>STGEEVVIAGMSGKLPESENLQEFWDNLIGGVDMVTDDDRRWKAGLYGLPRRSGKLKDLSRFDASFFGVHPKQAHTMDPQLRLLLEVTYEAIVDGGINPDSLRGTHTGVWVGVSGSETSEALSRDPETLVGYSMVGCQRAMMANRLSFFFDFRGPSIALDTACSSSLMALQNAYQAIHSGQCPAAIVGGINVLLKPNTSVQFLRLGMLSPEGTCKAFDTAGNGYCRSEGVVAVLLTKKSLARRVYATILNAGTNTDGFKEQGVTFPSGDIQEQLIRSLYQSAGVAPESFEYIEAHGTGTKVGDPQELNGITRALCATRQEPLLIGSTKSNMGHPEPASGLAALAKVLLSLEHGLWAPNLHFHSPNPEIPALLDGRLQVVDQPLPVRGGNVGINSFGFGGSNVHIILRPNTQPPPAPAPHATLPRLLRASGRTPEAVQKLLEQGLRHSQDLAFLSMLNDIAAVPATAMPFRGYAVLGGERGGPEVQQVPAGERPLWFICSGMGTQWRGMGLSLMRLDRFRDSILRSDEAVKPFGLKVSQLLLSTDESTFDDIVHSFVSLTAIQIGLIDLLSCMGLRPDGIVGHSLGEVACGYADGCLSQEEAVLAAYWRGQCIKEAHLPPGAMAAVGLSWEECKQRCPP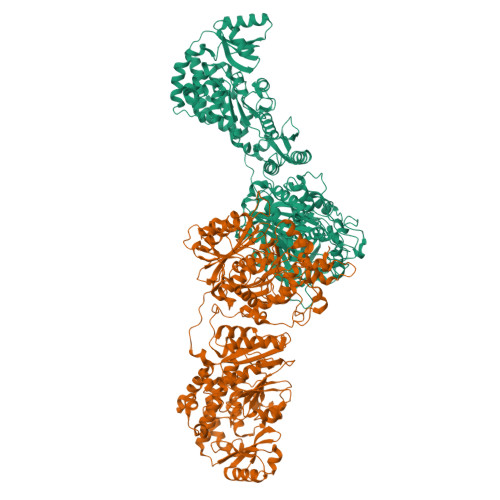GVVPACHNSKDTVTISGPQAPVFEFVEQLRKEGVFAKEVRTGGMAFHSYFMEAIAPPLLQELKKVIREPKPRSARWLSTSIPEAQWHSSLARTSSAEYNVNNLVSPVLFQEALWHVPEHAVVLEIAPHALLQAVLKRGLKPSCTIIPLMKKDHRDNLEFFLAGIGRLHLSGIDANPNALFPPVEFPAPRGTPLISPLIKWDHSLAWDVPAAEDFPNGSGSPSAAIYNIDTSSESPDHYLVDHTLDGRVLFPATGYLSIVWKTLARALGLGVEQLPVVFEDVVLHQATILPKTGTVSLEVRLLEASRAFEVSENGNLVVSGKVYQWDD[4x]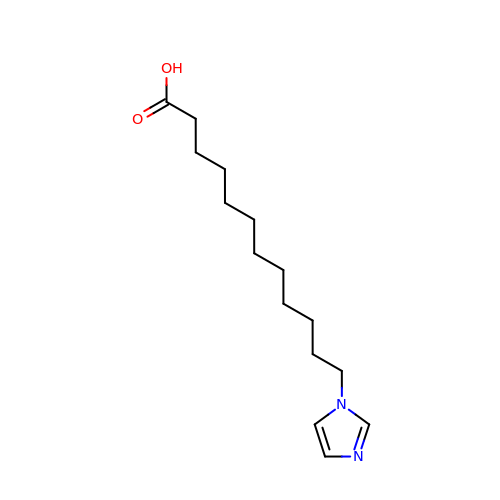12-(1H-imidazol-1-yl)dodecanoic acid | C15 H26 N2 O2 | XMSOPSLXOAQSRQ-UHFFFAOYSA-N> MSLQGIHLSDLSYKHAILKESQYTIKRDVGTTTAVTPSSLQQEITLLCGEILYAKHADYKYAAEIGIQYISTALGSERVQQILRNSGSEVQVVLTRTYSLGKIKNNKGEDLQMLDIHGVEKSWVEEIDKEARKTMATLLKESSGNIPQNQRPSAPDTPIILLCVGALIFTKLASTIEVGLETTVRRANRVLSDALKRYPRMDIPKIARSFYDLFEQKVYHRSLFIEYGKALGSSSTGSKAESLFVNIFMQAYGAGQTMLRWGVIARSSNNIMLGHVSVQAELKQVTEVYDLVREMGPESGLLHLRQSPKAGLLSLANCPNFASVVLGNASGLGIIGMYRGRVPNTELFSAAESYAKSLKESNKINFSSLGLTDEEKE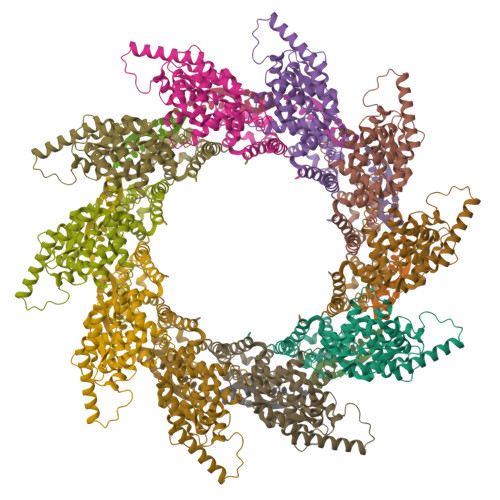AAEHFLNVSDDSQNDYE> MSGFNFGGTGAPTGGFTFGTAKTATTTPATGFSFSTSGTGGFNFGAPFQPATSTPSTGLFSLATQTPATQTTGFTFGTATLASGGTGFSLGIGASKLNLSNTAATPAMANPSGFGLGSSNLTNAISSTVTSSQGTAPTGFVFGPSTTSVAPATTSGGFSFTGGSTAQPSGFNIGSAGNSAQPTAPATLPFTPATPAATTAGATQPAAPTPTATITSTGPSLFASIATAPTS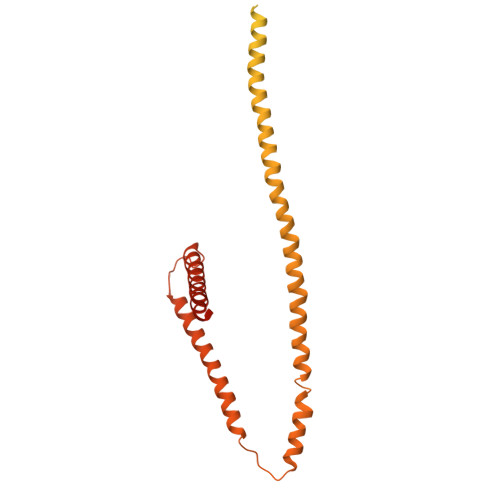SATTGLSLCTPVTTAGAPTAGTQGFSLKAPGAASGTSTTTSTAATATATTTSSSSTTGFALNLKPLAPAGIPSNTAAAVTAPPGPGAAAGAAASSAMTYAQLESLINKWSLELEDQERHFLQQATQVNAWDRTLIENGEKITSLHREVEKVKLDQKRLDQELDFILSQQKELEDLLSPLEELVKEQSGTIYLQHADEEREKTYKLAENIDAQLKRMAQDLKDIIEHLNTSGAPADTSDPLQQICKILNAHMDSLQWIDQNSALLQRKVEEVTKVCEGRRKEQERSFRITFD> DKDLERDTFSDFTFPEYYSTARVMGGLKNGVLYQGNIQISEYNFLEGSVSLPRFSKPVLIVGQKNLNRAFNGDQVIVELLPQSEWKAPSSIVLDSEHFDVNDNPDIEAGDDDDNNESSSNTTVISDKQRRLLAKDAMIAQRSKKIQPTAKVVYIQRRSWRQYVGQLAPSSVDPQSSSTQNVFVILMDKCLPKVRIRTRRAAELLDKRIVISIDSWPTTHKYPLGHFVRDLGTIESAQAETEALLLEHDVEYRPFSKKVLECLPAEGHDWKAPTKLDDPEAVSKDPLLTKRKDLRDKLICSIDPPGCVDINDALHAKKLPNGNWEVGVHIADVTHFVKPGTALDAEGAARGTSVYLVDKRIDMLPMLLGTDLCSLKPYVDRFAFSVIWELDDSANIVNVNFMKSVIRSREAFSYEQAQLRIDDKTQNDELTMGMRALLKLSVKLKQKRLEAGALNLASPEVKVHMDSETSDPNEVEIKKLLATNSLVEEFMLLANISVARKIYDAFPQTAMLRRHAAPPSTNFEILNEMLNTRKNMSISLESSKALADSLDRCVDPEDPYFNTLVRIMSTRCMMAAQYFYSGAYSYPDFRHYGLAVDIYTHFTSPIRRYCDVVAHRQLAGAIGYEPLSLTHRDKNKMDMICRNINRKHRNAQFAGRASIEYYVGQVMRNNESTETGYVIKVFNNGIVVLVPKFGVEGLIRLDNLTEDPNSAAFDEVEYKLTF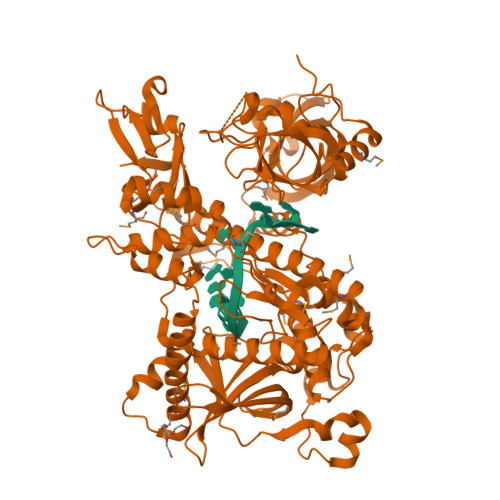VPTNSDKPRDVYVFDKVEVQVRSVMDPITSKRKAELLLK The DAP pathway commences with a condensation reaction between l-aspartate semialdehyde (ASA) and pyruvate to form (4S)−4-hydroxy-2,3,4,5-tetrahydro-(2S)-dipicolinic acid (HTPA), catalysed by HTPA synthase (EC 4.2.1.52), also known as dihydrodipicolinate synthase (DHDPS). Lysine regulates flux through the pathway by binding allosterically to DHDPS and inhibiting the enzyme. Thus, DHDPS catalyses the rate-limiting step of the DAP pathway. AtDHDPS enzymes exist as homotetramers, with the active site located within the (β/α)8-barrel and the allosteric cleft in the tight-dimer interface located in the interior of the structure (Griffin et al., 2012; Hall et al., 2021).

To probe the molecular determinants for inhibition, recombinant AtDHDPS1 was co-crystallised with MBDTA-2 using the same crystallisation conditions as for the apo enzyme with the addition of inhibitor. Diffraction data were obtained at a maximal resolution of 2.29 Å, phases solved by molecular replacement and repeating rounds of model building and refinement were performed that allowed us to generate an atomic inhibitor-bound model. Closer inspection of the crystal structure revealed the presence of four MBDTA-2 molecules bound at the centre of the homotetrameric protein, in antiparallel pairs with each molecule, which were stabilised by interactions across three of the monomers. Interestingly, this pocket, albeit distinct to the lysine binding site, shares two residues with it, namely W116 and E147. Specifically, the methoxy group of MBDTA-2 interacts with W116, E147, and H150 from chain B, while the pendant carboxylic acid interacts with S115 from chain A as well as H150 and Q154 from chain C. Additionally, we observed that upon binding, MBDTA-2 forces D117 to adopt a different rotamer conformation, which in turn, results in W116 assuming a different conformation. It must be noted that the four MBDTA-2 molecules were present with 50% occupancy. Consequently, each of the two moving residues, D117 and W116, adopt two distinct rotamer conformations, one of the apo- and ligand-bound states of AtDHDPS1. Given that no major rotamer changes or movement of catalytically important residues were noted, the exact mechanism of inhibition remains elusive. Moreover, an alignment of the primary structure of several DHDPS enzymes from plant species indicates that the residues involved in MBDTA-2 binding are highly conserved across both monocotyledons and dicotyledons and therefore should allow for broad-spectrum inhibition.

>MHHHHHHGKPALEVLFQGPGSMRSLEDKNRTNTDDIRSLRVITAIKTPYLPDGRFDLQAYDDLVNTQIENGAEGVIVGGTTGEGQLMSWDEHIMLIGHTVNCFGGRIKVIGNTGSNSTREAIHATEQGFAMGMHGALHINPYYGKTSIEGMNAHFQTVLHMGPTIIYNVPGRTCQDIPPQVIFKLSQNPNMAGVKECVGNNRVEEYTEKGIVVWSGNDDQCHDSRWDHGATGVISVTSNLVPGLMRKLMFEGRNSALNAKLLPLMDWLFQEPNPIGVNTALAQLGVARPVFRLPYVPLPLSKRIEFVKLVKEIGREHFVGDRDVQVLDDDDFILIGRY[2x]> 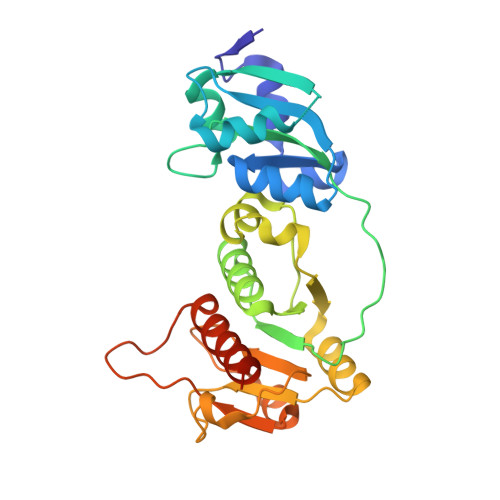MRITSTANPRIKELARLLERKHRDSQRRFLIEGAREIERALQAGIELEQALVWEGGLNPEEQQVYAALGRVGRLALLEVSEAVLKKLSVRDNPAGLIALARMPERTLEEYRPSPDALILVAVGLEKPGNLGAVLRSADAAGAEAVLVAGGVDLYSPQVIRNSTGVVFSLRTLAASESEVLDWIKQHNLPLVATTPHAEALYWEANLRPPVAIAVGPEHEGLRAAWLEAAQTQVRIPMQGQADSLNVSVSAALLLYEALRQRLLRDRLTKTHSTL>MEPVIIGALILDVHAKPSTTPISGTTVPGQVLFAPGGVARNVADCIFKLGITPFMIGTLGLDGPANVLLKEWKLSMKGILRREDISTPIVSLVYDTNGEVAAGVAGVDAVENFLTPEWIQRFEYNISSARLLMVDANLSSLALEASCKLAAESSVPVWFEPVSVTKSQRIASIAKYVTIVSPNQDELIAMANALCAKNLFHPFRSDENKLSIEDMFRALKPAILVLLKNGVKVVIVTLGSNGALLCSKGNPKKALNIDRKFLRSGEVFKRVQSVCSPN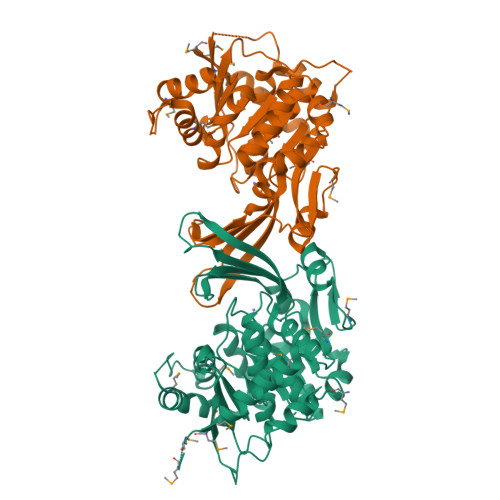RFSELGSNRSPSLFAMHFPTIPAKVKKLTGAGDCLVGGTVASLSDGLDLIQSLAVGIASAKAAVESDDNVPPEFKLDLISGDAELVYNGAKMLMVHQSML[2x]>AAQPAEECMHASGENYDGKISKTMSGLECQAWDSQSPHAHGYIPSKFPNKNLKKNYCRNPDRELRPWCFTTDPNKRWELCDIPRCTT[2x];> GSEELQGLKDDVEKLTADAELQRLKNERHEEAELERLKSERHDHDKKEAERKAL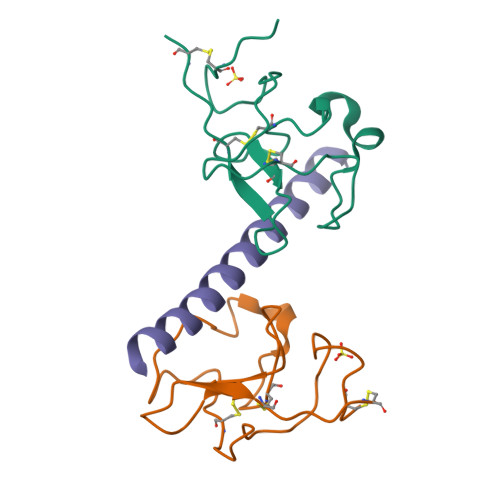EDKLADKQEHLNGALRYINEKEA> XSLSDKDKAAVRALWSKIGKSSDAIGNDALSRMIVVYPQTKIYFSHWPDVTPGSPNIKAHGKKVMGGIALAVSKIDDLKTGLMELSEQHAYKLRVDPSNFKILNHCILVVISTMFPK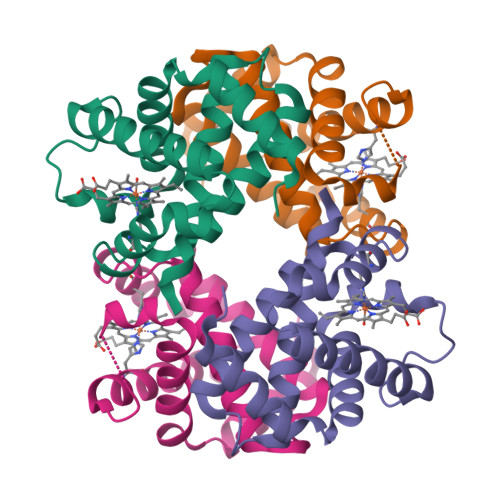EFTPEAHVSLDKFLSGVALALAERYR;> VEWTDKERSIISDIFSHMDYDDIGPKALSRCLVVYPWTQRYFSGFGNLYNAEGIMSNANVAAHGIKVLHGLDRGMKNMDNIADAYTDLSTLHSEKLHVDPDNFKLLSDCITIVLAAKMGHAFTAETQGAFQKFLAAVVSALGKQYH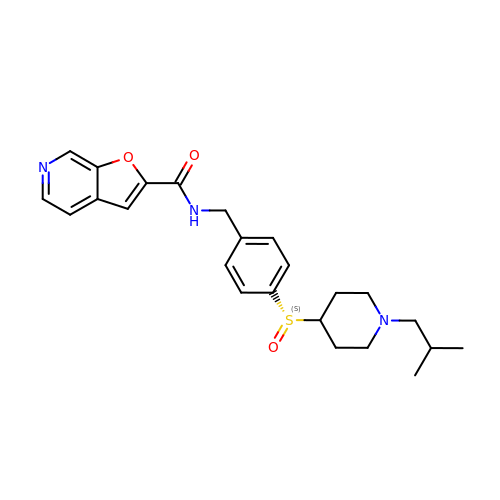N-(4-{(S)-[1-(2-methylpropyl)piperidin-4-yl]sulfinyl}benzyl)furo[2,3-c]pyridine-2-carboxamide | C24 H29 N3 O3 S | CIUHVWRNTOWXDH-WJOKGBTCSA-N>[4x]AIAMTHPDISVDVLVIGAGPTGLGAAKRLNQIDGPSWMIVDSNETPGGLASTDVTPEGFLYDVGGHVIFSHYKYFDDCLDEALPKEDDWYTHQRISYVRCQGQWVPYPFQNNISMLPKEEQVKCIDGMIDAALEARVANTKPKTFDEWIVRMMGTGIADLFMRPYNFKVWAVPTTKMQCAWLGERVAAPNLKAVTTNVILGKTAGNWGPNATFRFPARGGTGGIWIAVANTLPKEKTRFGEKGKVTKVNANNKTVTLQDGTTIGYKKLVSTMAVDFLA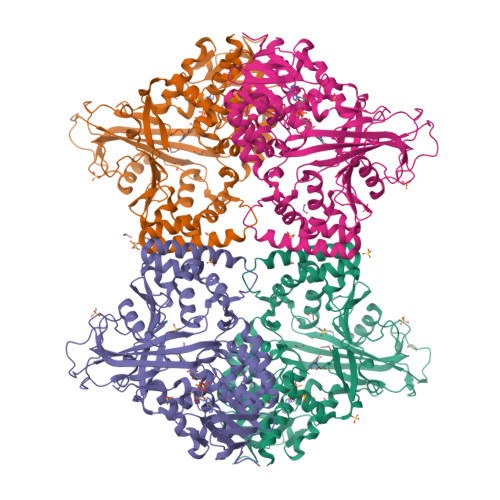EAMNDQELVGLTKQLFYSSTHVIGVGVRGSRPERIGDKCWLAFPEDNCPFYRATIFSNYSPYNQPEASAALPTMQLADGSRPQSTEAKEGPYWSIMLEVSESSMKPVNQETILADCIQGLVNTEMLKPTDEIVSTYHRRFDHGYPTPTLEREGTLTQILPKLQDKDIWSRGRFGSWRYEVGNQDHSFMLGVEAVDNIVNGAVELTLNYPDFVNGRQNTERRLVDGAQVFAKSKAQ> MAHHHHHHMSNNTIQAYAAMQAGEKLVPYKFDAGELQPHQVEVKVEYCGLCHSDISVLNNEWHSTVYPVVAGHEIIGRIVALGSEAKGLQIGQRVGIGWTAESCQACDECIGGQQVLCTGENIATIVGHAGGFADKVRAGWQWAIPLPEDLDPESAGPLLCGGITVFDPLLKHKIQATHHVGVIGIGGLGHIAIKLLKAWGCEITAFSSNPDKTEELKAMGADHVVNSRDTEAVKAQKGKFDLLLSTVNVTLNWRAFISTLAPNGSLHFLGLTLEPVPVSVGSLIDGAKSVTGSPTGSPAALRQLLKFAARKKIAPQ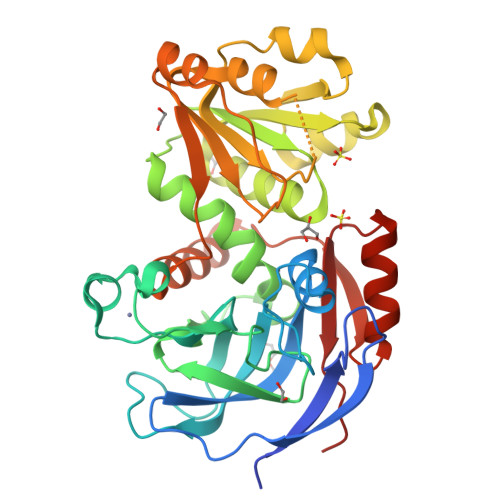IELFPMSQLNEAIERLHSGQARYRIVLKADFAE> MVDREWVLKIAKLARLELKEEEIEVFQKQLSDILDFIDQLKELDTENVEPYIQEFEETPMREDEPHPSLDREKALMN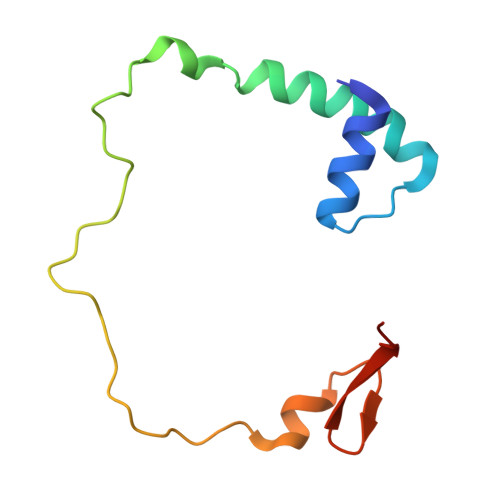APERKDGFFVVPRVVEV>[4x]TPASGALLQQMNLASQSLNYELSFISINKQ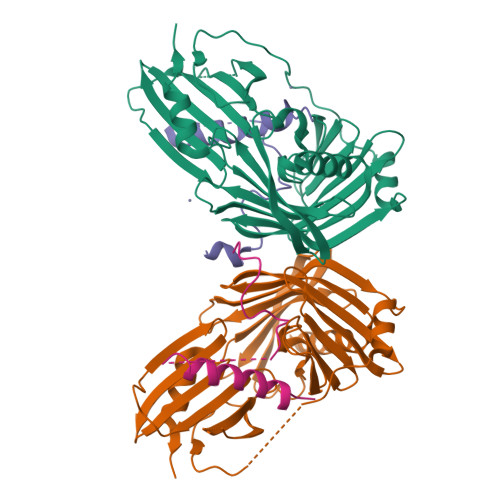GVESLRYRHARLDNRPLAQLLQMDGPRREVVQRGNEISYFEPGLEPFTLNGDYIVDSLPSLIYTDFKRLSPYYDFISVGRTRIADRLCEVIRVVARDGTRYSYIVWMDTESKLPMRVDLLDRDGETLEQFRVIAFNVNQDISSSMQTLAKANLPPLLSVPVGEKAKFSWTPTWLPQGFSEVSSSRRPLPTMDNMPIESRLYSDGLFSFSVNVNRATPSSTDQMLRTGRRTVSTSVRDNAEITIVGELPPQTAKRIAENIKFGAAQ;>YNGQSETSQQPETPVFNTLPMMGKASPVSLGVPSEATANNGQQQQVQEQRRRINAMLQDYELQRRLHSEQLQFEQAQTQQAAVQVPGIQTLGTQSQ[4x]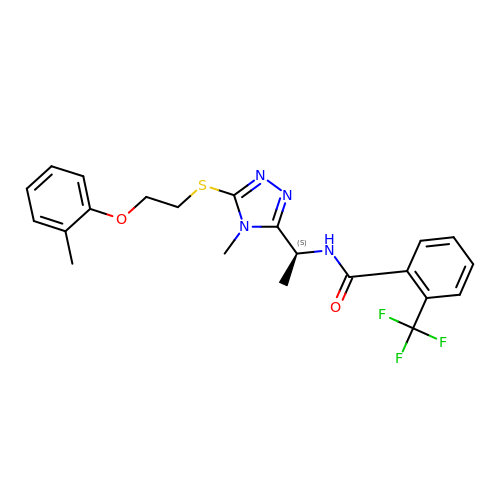N-[1-(4-methyl-5-{[2-(2-methylphenoxy)ethyl]sulfanyl}-4H-1,2,4-triazol-3-yl)ethyl]-2-(trifluoromethyl)benzamide | C22 H23 F3 N4 O2 S | AERPCBWEQRGXHO-HNNXBMFYSA-N>GSHMPETLVTVRRIEAQLGARVGVAVLDTGSGRSWEGYRADERFPMASTFKVLACGALLSRVDAGQEDLDRRIRYTQDELVTYSPVTEKHLDDGMTLRALCEATITTSDNTAANLILEALGGPKALTRFLRAIGDPVTRLDRWETALNEATPGDVRDTTTPRAMAATLRTLLLGDALTPASRQQLIAWLEANQVGGPLLRAGLPAGWRIGDKTGAGGRGTRGIVAIVWPPGRAPLIAAVYLTESEASMDERNAAIAEIGAALVKHW[2x]

The TEM-1 β-lactamase model system has been extensively used to study protein evolution. β-lactamases are a class of enzymes that are produced by bacteria in order to provide resistance to bactericidal β-lactam antibiotics through hydrolysis of their core β-lactam ring. We apply EVcouplings to computationally design variants of the model protein TEM-1 β-lactamase. To examine the structural effects of these mutations, we obtained X-ray crystal structures of designs 80.a, 80.b, and 70.a. Aligning these structures in 3D to a published WT TEM-1 structure (PDB: 1XPB34) revealed that all three have nearly identical Cα backbones to WT TEM-1 (0.26–0.61 Å RMSD over all Cα atoms).

Most notably, the 70.a design, which contains 88 mutations relative to WT TEM-1, had a ~32-fold increased MIC of the monobactam β-lactam antibiotic aztreonam, a 16-fold increased MIC of ceftazidime, an 8-fold increased MIC of cefazolin, and a 4-fold increased MIC of cephalothin. All of the designs that enabled resistance to ampicillin in the biological assays had a similar catalytic efficiency (kcat/KM) to WT TEM-1. This includes the 70.a design with 84 amino acid differences relative to any known protein. We also searched for local structural changes by examining differences in all pairwise distances between residues, which showed small changes in a one looped region for all three structures (positions 255–257) and in a second loop of 70.a (positions 53–55). The G251W mutation, which was present in both 70.a and opt.b, stood out due to multiple studies that describe it as negatively impacting fitness in WT TEM-125,51. In the 70.a structure, new local interactions between mutated residues W251 and R230 and non-mutated residue E212 may contribute to maintaining β-lactamase structure and function. In summary, (1) 70.a contains many point mutations that have been described in the literature as compensatory, (2) these mutations combined with G251W have some of the highest predicted fitness effects, and (3) structural analysis suggests that local interactions between W251 and R230 (a mutation in 70.a F230R) may be important for maintaining function. However, the other functional designs contain amino acid changes that exhibit fitness defects in WT TEM-1; 80.a has two amino acid changes that show fitness defects, 80.b has four, 70.a has 11 and opt.b has 28. To investigate the structural basis for the increased Tm (80.a had a 24 °C increase relative to WT TEM-1, 80.b had a 18 °C increase, and 70.a had a 6.3 °C increase), we tallied the total number of hydrogen bonds and the number of atom pairs in contact (1.7–4 Å) in each structure. There are five shared mutations near the active site that are in three designs (M69A, E104T, P167T, E168A, E240G) that may contribute to this increased resistance.> MIRWGLIGASTIAREWVIGAIRAAGGEVVSVMSSSAERGEAYAAENGIAKAVTSVDDLVGDPDVDAVYISTTNELHHGQALAAIRAGKHVLCEKPLAMNLNDGCEMVLKACE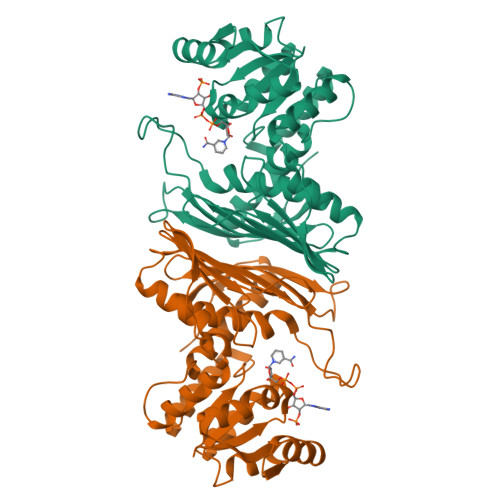AGVVLGTNHHLRNAATHRAMREAIAAGRIGRPIAARVFHAVYLPPHLQGWRLDKPEAGGGVILDITVHDADTLRFVLNDDPIEAVAISHSAGMGKEGLEDGVMGVLRFRSGVIAQFHDAFTTKFAETGLEVHGTAGSLIGRNVMTQRPVGTVVLRNEEGESELPLDHRNLYETAIAAFHSAIGGNGRPSASGEDGVWSLATGLAVVKAAATGGAVEIETGL2-(5-chloranyl-1~{H}-indol-3-yl)ethanamine 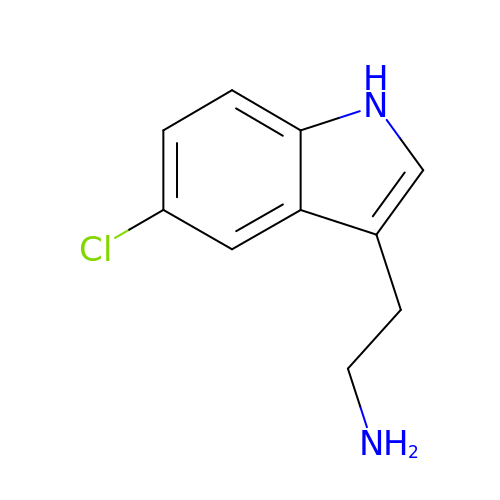| C10 H11 Cl N2 | FVQKQPVVCKOWLM-UHFFFAOYSA-N> TKT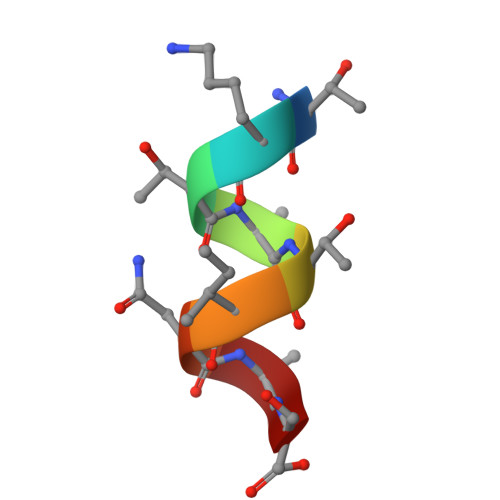ATINAS> MTTVPDLESDSFHVDWYRTYAELRETAPVTPVRFLGQDAWLVTGYDEAKAALSDLRLSSDPKKKYPGVEVEFPAYLGFPEDVRNYFATNMGTSDPPTHTRLRKLVSQEFTVRRVEAMRPRVEQITAELLDEVGDSGVV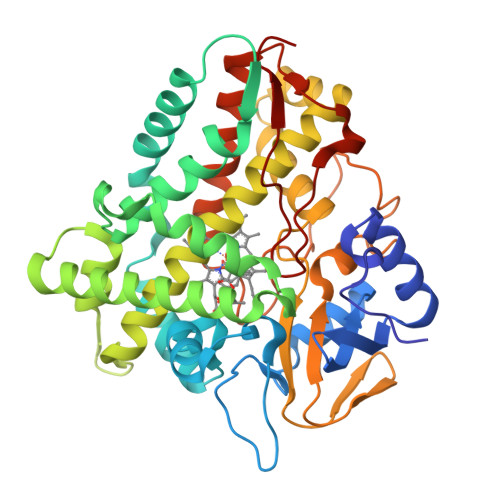DIVDRFAHPLPIKVICELLGVDEKYRGEFGRWSSEILVMDPERAEQRGQAAREVVNFILDLVERRRTEPGDDLLSALIRVQDDDDGRLSADELTSIALVLLLAGFEASVSLIGIGTYLLLTHPDQLALVRRDPSALPNAVEEILRYIAPPETTTRFAAEEVEIGGVAIPQYSTVLVANGAANRDPKQFPDPHRFDVTRDTRGHLSFGQGIHFCMGRPLAKLEGEVALRALFGRFPALSLGIDADDVVWRRSLLLRGIDHLPVRLDG> MEYIIKNGFVYCPLNGVDGEKMDICVKDGKIVESVSDSAKVIDASGKIVMPGGVDPHSHIAGAKVNVGRMYRPEDSKRDAEKFKGGRAGSGFSVPSTFMTGYRYAQMGYTTAMEAAMPPLLARHTHEEFHDTPIIDHAAYPLFGNNWFVMEYLKEGDVDACAAYASWLLRATKGYTIKIVNPAGTEAWGWGGNVHGIYDPAPYFDITPAEIIKGLAEVNEKLQLPHSIHLHCNDLGHPGNYETTLASFDVPKNIKPNPATGSRDTVLYATHVQFHSYGGTTWRDFVSEAPKIADYVNKNDHIVIDVGQITLDETTTMTADGPMEYDLHSLNGLKWANCDVELETGSGVVPFIYSARAPVPAVQWAIGMELFLLIDNPEKVCLTTDSPNAGPFTRYPRVIAWLMSNKYRMNLIEGELHKWAQRKSTVATIDREYTFSEIAQITRATSAKVLGLSDTKGHLGVGADADIAVYDINPETVDPSAEYMAIEEAFSRAACVLKDGEIVVKDGEVVASPHGRTYWVDTQVDESIYSEVLANVESKFKQYYSVNFANYPVQDDYLPKSAPVKGVML;> MEYVKNVVCPFCGTLCDDIICKVEGNEIVGTINACRIGHSKFVHAEGAMRYKKPLIRKNGEFVEVSYDEAIDKAAKILAESKRPLMYGWSCTECEAQAVGVELAEEAGAVIDNTASVCHGPSVLALQDVGYPICTFGEVKNRADVVVYWGCNPMHAHPRHMSRNVFARGFFRERGRSDRTLIVVDPRKTDSAKLADIHLQLDFDRDYELLDAM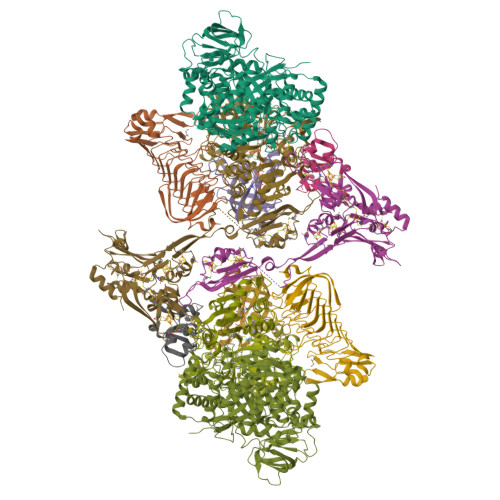RACLLGHEILYDEVAGVPREQIEEAVEVLKNAQFGILFFGMGITHSRGKHRNIDTAIMMVQDLNDYAKWTLIPMRGHYNVTGFNQVCTWESGYPYCVDFSGGEPRYNPGETGANDLLQNREADAMMVIASDPGAHFPQRALERMAEIPVIAIEPHRTPTTEMADIIIPPAIVGMEAEGTAYRMEGVPIRMKKVVDSDLLSDREILERLLEKVREYKASK;> MSEIILTPKEQPEVPLEAPNIKPDVFAGKSIEEIKNIQIMHGNEVVKLGDFFEVSGEPADAPEDIKIIIDGDVYNTKRIGQEMTAGEIIVRGNVNMYVGAGMKGGKITVEGNAGSWAGQDMRGGEIEILGDAGDYVGSSYRGDWRGMSGGTITVHGNADNEIGEYMNGGKIIIKGDVNIMPGIHMNNGLIIIEGNVVARAGGEMAGGTIVVKGMMQEFLAGFKYLGVEKDIEVDGEELPGAFYKFEGDHAIKGAKGIVYAAVGCNGHIAP;> MRVILNTGRTIWQGQAIESGKDLKMYVDAAAIIQMNPEMMKQLGIAEGDNVKVISEYGDVVVKAVEAKEPLPEGMVYIPMGPWANRVIRPYTDSTATPSFKNIPVEIIPTDEEVLDMPTLMKVYGKVGQI;> METTEVIEGKNITVERTGEENRRLIFQDCLCAVCGLCGEICPVSAIEVNPTGAMVRTEQEKSKIAIDENKCVLCGMCSSICPFQALDLQIDGTSIKELAEYPKIIKSAEIDDETCIQCKACETACPQDAITITRELPERKDLVTGEIEIDKDTCIYCGMCEEMCPVDAIEIDHQTPSSASPVVATDIRVDEDKCVHCGICKRICPVDAIMQVCRICPYGEYEIKTPEVTGTSYIDPELCVNCGWCQEICPVDAATVTKPFEGELIIDQDTCQACETCVMVCPCNVLSFPKPEKPGEKTTKLHKDERFCIYCGACERSCPVTAITVKRNRINTTPIRSKAWKNAFDSLLK;> MAIGLKAYPELCHGCGNCVIACPVNALRSPEVAGGKGPTDDVEIIMIVEDGVVNIKNPDLCGKCGTCVESCPVDAIRLEELE> GVGISTGTFNNQTEFKFLENGWVEITANSSRLVHLNMPESENYRRVVVNNMDKTAVNGNMALDDIHAQIVTPWSLVDANAWGVWFNPGDWQLIVNTMSELHLVSFEQ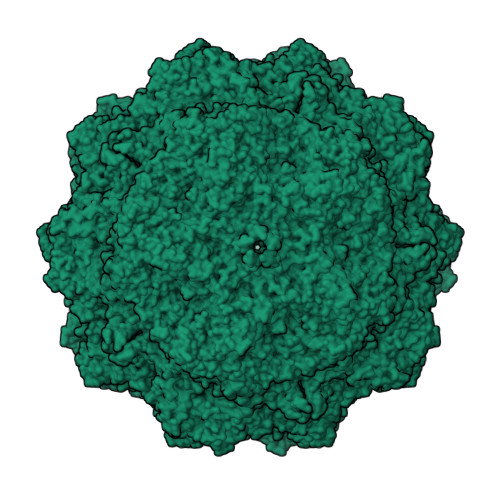EIFNVVLKTVSESATQPPTKVYNNDLTASLMVALDSNNTMPFTPAAMRSETLGFYPWKPTIPTPWRYYFQWDRTLIPSHTGTSGTPTNIYHGTDPDDVQFYTIENSVPVHLLRTGDEFATGTFFFDCKPCRLTHTWQTNRALGLPPFLNSLPQSEGATNFGDIGVQQDKRRGVTQMGNTNYITEATIMRPAEVGYSAPYYSFEASTQGPFKTPIAAGRGGAQTDENQAADGNPRYAFGRQHGQKTTTTGETPERFTYIAHQDTGRYPEGDWIQNINFNLPVTNDNVLLPTDPIGGKTGINYTNIFNTYGPLTALNNVPPVYPNGQIWDKEFDTDLKPRLHVNAPFVCQNNCPGQLFVKVAPNLTNEYDPDASANMSRIVTYSDFWWKGKLVFKAKLRASHTWNPIQQMSINVDNQFNYVPSNIGGMKIVYEKSQLAPRKLY> MSSNRVLDLFKPFESFLPEVIAPERKVPYNQKLIWTGVSLLIFLILGQIPLYGIVSSETSDPLYWLRAMLASNRGTLLELGVSPIITSSMIFQFLQGTQLLQIRPESKQDRELFQIAQKVCAIILILGQALVVVMTGNYGAPSDLGLPICLLLIFQLMFASLIVMLLDELLSKGYGLGSGISLFTATNIAEQIFWRAFAPTTVNSGRGKEFEGAVIAFFHLLAVRKDKKRALVEAFYRTNLPNMFQVLMTVAIFLFVLYLQGFRYELPIRSTKVRGQIGIYPIKLFYTSNTPIMLQSALTSNIFLISQILFQKYPTNPLIRLIGVWGIRPGTQGPQMALSGLAYYIQPLMSLSEALLDPIKTIVYITFVLGSCAVFSKTWIEISGTSPRDIAKQFKDQGMVINGKRETSIYRELKKIIPTAAAFGGATIGALSVGSDLLGTLGSGASILMATTTIYGYYEAAAKEGGFTKNLVPGFSDLM;> MSSPTPPGGQRTLQKRKQGSSQKVAASAPKKNTNSNNSILKIYSDEATGLRVDPLVVLFLAVGFIFSVVALHVISKVAGKLF;> MARASEKGEEKKQSNNQVEKLVEAPVEFVREGTQFLAKCKKPDLKEYTKIVKAVGIGFIAVGIIGYAIKLIHIPIRYVIV;> GGSGGSGGSGGSGGSPTNYEYDEASETWPSFILTGLLMVVGPMTLLQIYQIFFGANAEDGNSGKSKEFNEEVFKNLNEEYTSDEIKQFRRKFDKNSNKKSKIWSRRNIIIIVGWILVAILLQRINSNDAIKDAATKLFDPYEILGISTSASDRDIKSAYRKLSVKFHPDKLAKGLTPDEKSVMEETYVQITKAYESLTDELVRQNYLKYGHPDGPQSTSHGIALPRFLVDGSASPLLVVCYVALLGLILPYFVSRWWARTQSYTKKGIHNVTASNFVSNLVNYKPSEIVTTDLILHWLSFAHEFKQFFPDLQPTDFEKLLQDHINRRDSGKLNNAKFRIVAKCHSLLHGLLDIACGFRNLDIALGAINTFKCIVQAVPLTPNCQILQLPNVDKEHFITKTGDIHTLGKLFTLEDAKIGEVLGIKDQAKLNETLRVASHIPNLKIIKADFLVPGENQVTPSSTPYISLKVLVRSAKQPLIPTSLIPEENLTEPQDFESQRDPFAMMSKQPLVPYSFAPFFPTKRRGSWCCLVSSQKDGKILQTPIIIEKLSYKNLNDDKDFFDKRIKMDLTKHEKFDINDWEIGTIKIPLGQPAPETVGDFFFRVIVKSTDYFTTDLDITMNMKVRDSPAVEQVEVYSEEDDEYSTDDDETESDDESDASDYTDIDTDTEAEDDESPEAGGATTASGTGENLYFQ;> MSEFNETKFSNNGTFFETEEPIVETKSISVYTPLIYVFILVVSLVMFASSYRKKQAKKISEQPSIFDENDAHDLYFQIKEMSENEKIHEKVLKAALLNRGAESVRRSLKLKELAPQINLLYKNGSIGEDYWKRFETEVKLIELEFKDTLQEAERLQPGWVQLFVMVCKEICFNQALSRRYQSILKRKEVCIKEWELKINNDGRLVN;> MVTLEYNANSK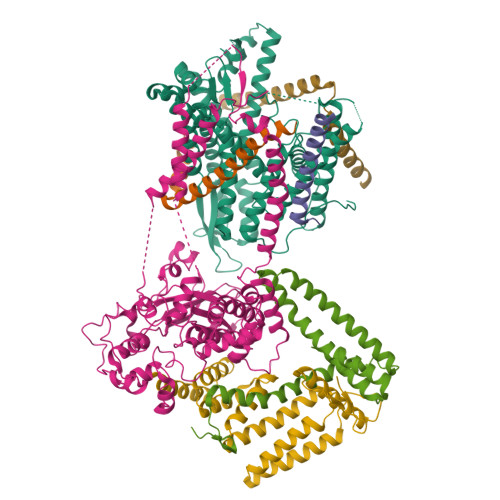LITASDAVVALSTETNIDQINVLTTSLIGETNPNFTPQPNEALSKMIKGLFESGMKNLQQKKLNEALKNVSLAIEMAQRKRAPWEAFAIQLPELHFMLRSKIDLCLILGKHLEALQDLDFLLGTGLIQPDVFVRKADCLLKLRQWEEARATCERGLALAPEDMKLRALLIETARNLAEYNGE> MPADNYHLARRRTLQVVVSSLLTEAGFESAEKASVETLTEMLQSYISEIGRSAKSYCEHTARTQPTLSD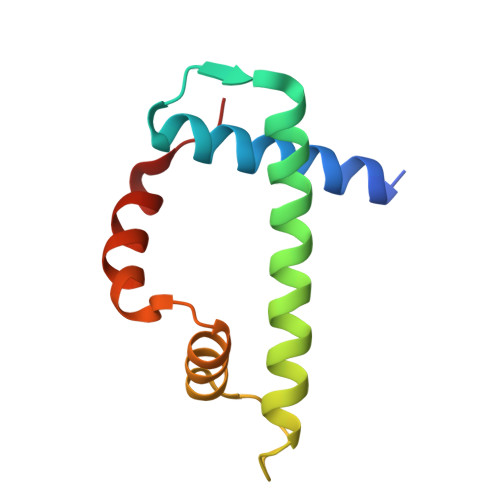IVVTLVEMGFNVDTLPAYAKRSQRMVIT> SNAMSKLPENFLWGGAVAAHQLEGGWQEGGKGISVADVMTAGRHGVAREITAGVLEGKYYPNHEAIDFYHHYKEDVKLFAEMGFKCFRTSIAWTRIFPKGDEAEPNEAGLQFYDDLFDECLKYGIEPVVTLSHFELPYHLVTEYGGFTNRKVIDFFVHFAEVCFRRYKDKVKYWMTFNEINNQANYQEDFAPFTNSGIVYKEGDDREAIMYQAAHYEL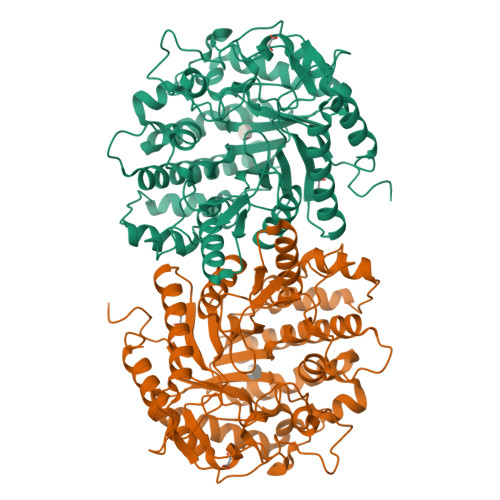VASARAVKIGHAINPNLNIGCMVAMCPIYPATCNPKDILMAQKAMQKRYYFADVHVHGFYPEHIFKYWERKAIKVDFTERDKKDLFEGTVDYIGFSYYMSFVIDAHRENNPYYDYLETEDLVKNPYVKASDWDWQIDPQGLRYALNWFTDMYHLPLFIVQNGFGAIDQVEADGMVHDDYRIDYLGAHIKEMIKAVDEDGVELMGYTPWGCIDLVSAGTGEMRKRYGFIYVDKDDEGKGTLKRSPKLSFNWYKEVIASNGDDI> TVLPKDI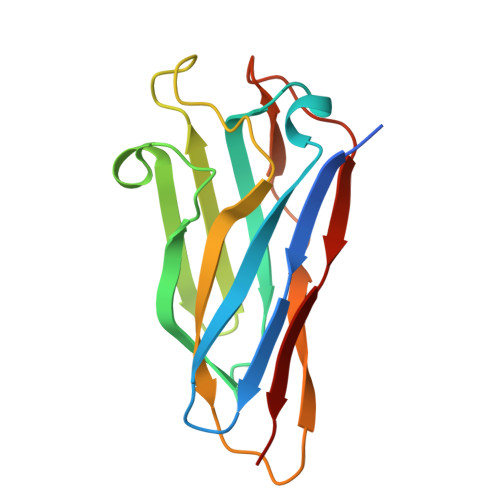PGDSLKVTVGTANGKPGDTVTVPVTFADVAKMKNVGTCNFYLGYDASLLEVVSVDAGPIVKNAAVNFSSSASNGTISFLFLDNTITDELITADGVFANIKFKLKSVTAKTTTPVTFKDGGAFGDGTMSKIASVTKTNGSVTIDP> APVAAYVDEVLNEVLVVPNINQSHPTTSNAAPVLDAAETGHTNKIQPEDTIETRYVQSSQTLDEMSVESFLGRSGCIHESVLDIVDNYNDQSFTKWNINLQEMAQIRRKFEMFTYARFDSEITMVPSVAAKDGHIGHIVMQYMYVPPGAPIPTTRDDYAWQSGTNASVFWQHGQPFPR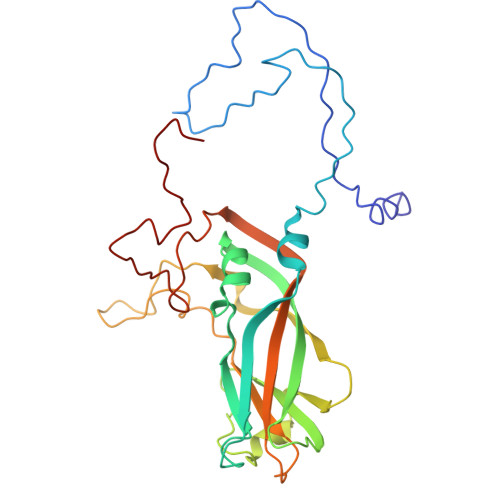FSLPFLSIASAYYMFYDGYDGDTYKSRYGTVVTNDMGTLCSRIVTSEQLHKVKVVTRIYHKAKHTKAWCPRPPRAVQYSHTHTTNYKLSSEVHNDVAIRPRTNLTTV>PKISLQIPIKLKSVLVDDWEYVTKDKKICRLPADVTVEMVLNKYEHEVSQELESPGSQSQLSEYCAGLKLYFDKCLGNMLLYRLERLQYDELLKKSSKDQKPLVPIRIYGAIHLLRLISVLPELISSTTMDLQSCQLLIKQTEDFLVWLLMHVDEYFNDKDPNRSDDALYVNTSSQYEGVALGM[2x];>EETLLELNNRIRVRKQDFTLPWEEYGELILENARKS[2x]

In Saccharomyces cerevisiae, reduced potassium dependency-3 (Rpd3) resides in two distinct histone deacetylase complexes, termed Rpd3S and Rpd3L1–3. The Rpd3S complex functions to repress transcriptional initiation within the coding region of genes during RNA polymerase II elongation by maintaining hypoacetylation. Rco1 recognizes unmodified H3K4 (H3K4me0) via its PHD1 domain and associates with Eaf3 to enhance the Eaf3–H3K36me3 interaction. In this study, we presented the structures of Eaf3MRG bound with Rco1PHD1–SID and H3K4me0 or with a fragment of Eaf7.

To address these unknowns, we identified a region within Eaf7 (aa 108–143) as the Eaf3MRG binding motif using GST pull-down assays and solved the structure of Eaf3MRG bound with Eaf7108–143 at a resolution of 2.40 Å. Residues 111–142 of Eaf7 are visible in the complex and adopt two helices (α1 and α2) connected by a long linker. Eaf7108–143 binds to Eaf3MRG mainly via hydrophobic interactions. α1 of Eaf7108–143 interacts with α3, α5 and α6 of Eaf3MRG mainly via hydrophobic interactions; the linker region of Eaf7 interacts with α3, α4, and α5 of Eaf3MRG via hydrophobic and hydrogen bonding interactions; α2 of Eaf7108–143 packs against α1 of Eaf3MRG. The main chain carbonyl group of Eaf7 Glu131 is hydrogen-bonded to Eaf3 Lys229, which forms an additional polar interaction with the side chain of Glu131. Consistently, mutagenesis and GST pull-down assays showed that L114A, I118A, R121A, D124A, and E131A of Eaf7108–143 slightly reduce the binding to Eaf3MRG, while F125A and L127A of Eaf7108–143 abolish the binding. In addition, R300A/R303E, V233E/W236D, and V233E/T240A of Eaf3MRG disrupt the binding to Eaf7108–143, suggesting that Eaf7108–143 and Rco1SID1–PHD bind to the same site on Eaf3MRG. Furthermore, ITC binding assay showed that SUMO–Eaf7108–143 binds to Eaf3MRG with a KD value of 1.0 μM but displays no binding toward the Eaf3MRG–Rco1PHD1–SID complex. Taken together, the structural analysis and binding data confirm that Eaf7108–143 and Rco1PHD1–SID bind to the same surface of Eaf3MRG. All MRG-binding ligands contain a common helix–linker–helix motif, such as α3–α4 of Rco1, α1–α2 of Eaf7, and α2–α3 of MRGBP. In addition, the solved structures confirm that Eaf7 and Rco1 bind to the same surface on Eaf3MRG, which complements our understanding of how Eaf3 resides in distinct histone modification complexes.> ID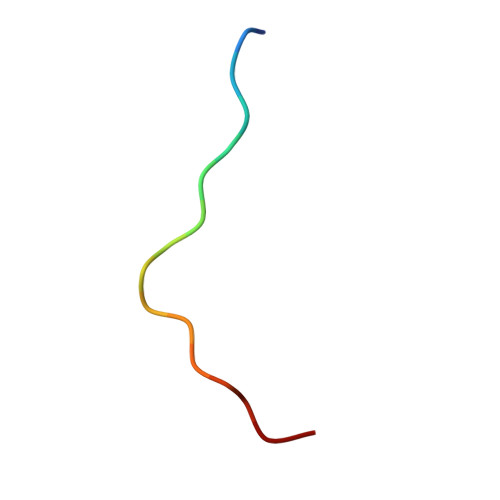RYEQVSKDFEFIKI>[2x]MAVLAESELGSEAQRERRKRILD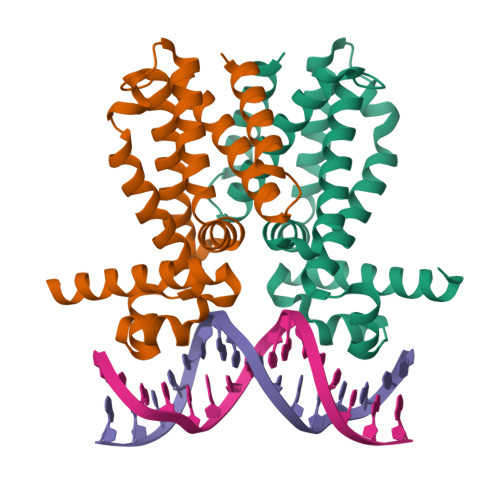ATMAIASKGGYEAVQMRAVADRADVAVGTLYRYFPSKVHLLVSALGREFSRIDAKTDRSAVAGATPFQRLNFMVGKLNRAMQRNPLLTEAMTRAYVFADASAASEVDQVEKLIDSMFARAMANGEPTEDQYHIARVISDVWLSNLLAWLTRRASATDVSKRLDLAVRLLIGDQDSAHHHHHH> MLKRKQSSRVEAQPVTDFGPDESLSDNADILWINKPWVHSLLRICAIISVISVCMNTPMTFEHYPPLQYVTFTLDTLLMFLYTAEMIAKMHIRGIVKGDSSYVKDRWCVFDGFMVFCLWVSLVLQVFEIADIVDQMSPWGMLRIPRPLIMIRAFRIYFRFELPRTRITNILKRSGEQIWSVSIFLLFFLLLYGILGVQMFGTFTYHCVVNDTKPGNVTWNSLAIPDTHCSPELEEGYQCPPGFKCMDLEDLGLSRQELGYSGFNEIGTSIFTVYEASSQEGWVFLMYRAIDSFPRWRSYFYFITLIFFLAWLVKNVFIAVIIETFAEIRVQFQQMWGTRSSTTSTATTQMFHEDAAGGWQLVAVDVNKPQGRAPACLQKMMRSSVFHMFILSMVTVDVIVAASNYYKGENFRRQYDEFYLAEVAFTVLFDLEALLKIWCLGFTGYISSSLHKFELLLVIGTTLHVYPDLYHSQFTYFQVLRVVRLIKISPALEDFVYKIFGPGKKLGSLVVFTASLLIVMSAISLQMFCFVEELDRFTTFPRAFMSMFQILTQEGWVDVMDQTLNAVGHMWAPLVAIYFILYHLFATLILLSLFVAVILDNLELDEDLKKLKQLKQSEANADTKEKLPLRLRIFEKFPNRPQMVKISKLPSDFTVPKIRESFMKQFIDRQQQDTCCLFRILPSTSSSSCDNPKRPTVEDNKYIDQKLRKSVFSIRARNLLEKETAVTKILRACTRQRMLSGSFEGQPAKERSILSVQHHIRQERRSLRHGSNSQRISRGKSLETLTQDHSNTVRYRNAQREDSEIKMIQEKKEQAEMKRKVQEEELRENHPYFDKPLFIVGREHRFRNFCRVVVRARFNASKTDPVTGAVKNTKYHQLYDLLGLVTYLDWVMITVTICSCISMMFESPFRRVMHAPTLQIAEYVFVIFMSIELNLKIMADGLFFTPTAVIRDFGGVMDIFIYLVSLIFLCWMPQNVPAESGAQLLMVLRCLRPLRIFKLVPQMRKVVRELFSGFKEIFLVSILLLTLMLVFASFGVQLFAGKLAKCNDPNIIRREDCNGIFRINVSVSKNLNLKLRPGEKKPGFWVPRVWANPRNFNFDNVGNAMLALFEVLSLKGWVEVRDVIIHRVGPIHGIYIHVFVFLGCMIGLTLFVGVVIANFNENKGTALLTVDQRRWEDLKSRLKIAQPLHLPPRPDNDGFRAKMYDITQHPFFKRTIALLVLAQSVLLSVKWDVEDPVTVPLATMSVVFTFIFVLEVTMKIIAMSPAGFWQSRRNRYDLLVTSLGVVWVVLHFALLNAYTYMMGACVIVFRFFSICGKHVTLKMLLLTVVVSMYKSFFIIVGMFLLLLCYAFAGVVLFGTVKYGENINRHANFSSAGKAITVLFRIVTGEDWNKIMHDCMVQPPFCTPDEFTYWATDCGNYAGALMYFCSFYVIIAYIMLNLLVAIIVENFSLFYSTEEDQLLSYNDLRHFQIIWNMVDDKREGVIPTFRVKFLL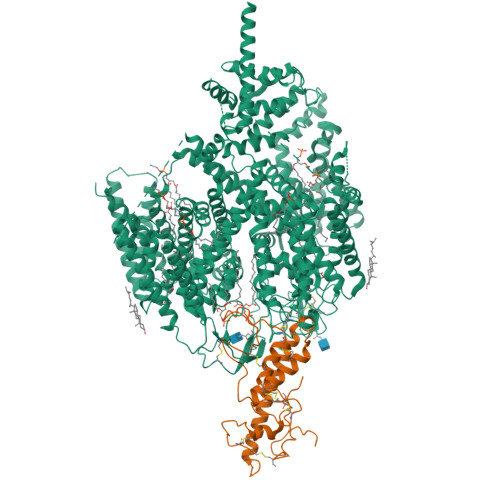RLLRGRLEVDLDKDKLLFKHMCYEMERLHNGGDVTFHDVLSMLSYRSVDIRKSLQLEELLAREQLEYTIEEEVAKQTIRMWLKKCLKRIRAKQQQSCSIIHSLRESQQQELSRFLNPPSIETTQPSEDTNANSQDHNTQPESSSQQQLLSPTLSDRGGSRQDAADTGKPQRKIGQWRLPSAPKPISHSVSSVNLRFGGRTTMKSVVCKMNPMPDTASCGSEVKKWWTRQLTVESDESGDDLLDI;> MTRGAWMCRQYDDGLKIWLAAPRENEKPFIDSERAQKWRLSLASLLFFTVLLSDHLWFCAEAKLTRTRDKEHHQQQQQQQQQQQQQQQQQQQQQQRQQQRQRQQQRQRQQEPSWPALLASMGESSPAAQAHRLLSASSSPTLPPSPGGGGGSKGNRGKNNRSRALFLGNSAKPVWRLETCYPQGASSGQCFTVESADAVCARNWSRGAAAGEEQSSRGSRPTPLWNLSDFYLSFCNSYTLWELFSGLSSPSTLNCSLDVVLTEGGEMTTCRQCIEAYQDYDHHAQEKYEEFESVLHKYLQSDEYSVKSCPEDCKIVYKAWLCSQYFEVTQFNCRKTIPCKQYCLEVQTRCPFILPDNDEVIYGGLSSFICTGLYETFLTNDEPECCDIRSEEQTAPRPKGTVDRRDSCPRTSLTVSSATRLCPGRLKLCVLVLILLHTVLTASAAQNSTGLGLGGLPTLEDNSTRED Bacteriophage T5, a representative member of the T5-like family of siphophages, serves as an excellent model for studying the assembly, infection, cell wall perforation, and DNA ejection mechanisms of this phage family. In this study, we used cryo-electron microscopy (cryo-EM) to determine the structures of mature T5 (a laboratory-adapted, fiberless T5 mutant) and urea-treated empty T5 (lacking the tip complex) at near-atomic resolutions. The T5 head comprises 775 copies of MCP gp8, arranged into 11 pentons and 120 hexons, forming an icosahedral shell with a triangle number (T) of 13. The T5 tail, which comprises 40 trimeric rings of the TTP and a distal tip complex, is connected to a unique five-fold vertex of the head by the connector complex.

We built atomic models for the portal, adaptor, and tail terminator of urea-treated empty T5. In contrast to the mature T5, the DNA and TMP are ejected in urea-treated empty T5, resulting in an empty head and an unoccupied tail tube. The release of the TMP and DNA in urea-treated T5 results in an empty tail and an empty head. A structural comparison of the connector complex between the two states revealed that the connector did not undergo any global conformational change. Structural comparisons of the portal, adaptor, and tail terminator proteins before and after DNA release indicated that no discernible conformational changes had occurred in these regions during infection. In the DNA-ejected state, once the interaction of the tail tip complex or baseplate with the host cell induces the release of TMP, the large space of the connector complex enables the passage of DNA. No significant differences were observed in the conformation of connector proteins before and after DNA release, and these proteins appear to be conserved across myophages and siphophages. However, T5 and DT57C lack a stopper in the connector complex, suggesting that the dodecameric adaptor may assume the stopper function, serving as a docking platform for the tail by binding to the tail terminator protein and ultimately completing the formation of the connector complex. Notably, the tip complex of the empty particle became detached for urea-treatment-induced reasons.

>MGFKSWITEKLNPGQRIIRDMEPVSHRTNRKPFTTGQAYSKIEILNRTANMVIDSAAECSYTVGDKYNIVTYANGVKTKTLDTLLNVRPNPFMDISTFRRLVVTDLLFEGCAYIYWDGTSLYHVPAALMQVEADANKFIKKFIFNNQINYRVDEIIFIKDNSYVCGTNSQISGQSRVATVIDSLEKRSKMLNFKEKFLDNGTVIGLILETDEILNKKLRERKQEELQLDYNPSTGQSSVLILDGGMKAKPYSQISSFKDLDFKEDIEGFNKSICLAFGVPQVLLDGGNNANIRPNIELFYYMTIIPMLNKLTSSLTFFFGYKITPNTKEVAALTPDKEAEAKHLTSLVNNGIITGNEARSELNLEPLDDEQMNKIRIPANVAGSATGVSGQEGGRPKGSTEGD[12x];>[12x]MQIITAEDYRLYGGLKRPELESGVEVMITAANALITSLLGMDDADAVDQLITTKPTRKKYFLSSPSATSVTKMTINDKEIDPEQYKLYSDGVILLKFNPPEGYMDVEYTQGGFNPMPEDLKLAACMLVDHWHKQDYRQARTIGGETVTFNNTKSGIPEHIRTIIEVYRRV> ATFTMNLPWSQGYYWYSGGAHSNTGSGYPYSSLD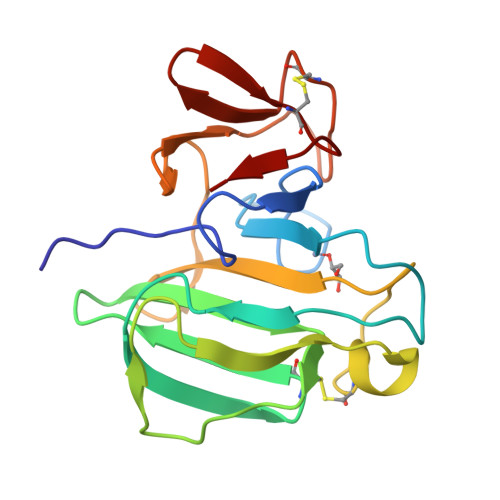FNNGSGGWGSNTPWVQAAHGGVITRFSSCNIRVTHSSGFATNYYHMSNLQYNNGDTVQPGTLLGRYANSYNQALCEGGQSSGPHVHFTLLQNGQQVSLHNRYISNYRIDVGNSNYDSNCNNFYFERNGRRTCAWRPLYR>[2x]MDLTNKNVIFVAALGGIGLDTSRELVKRNLKNFVILDRVENPTALAELKAINPKVNITFHTYDVTVPVAE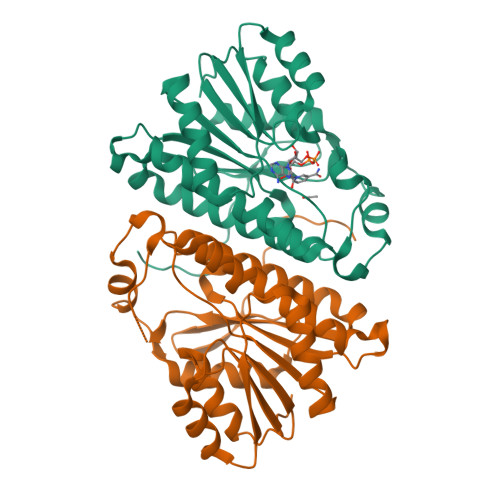SKKLLKKIFDQLKTVDILINGAGILDDHQIERTIAINFTGLVNVTTAILDFWDKRKGGPGGIIANICSVTGFNAIHQVPVYSASKAAVVSFTNSLAKLAPITGVTAYSINPGITRTPLVHTFNSWLDVEPRVAELLLSHPTQTSEQCGQNFVKAIEANKNGAIWKLDLGTLEAIEWTKHWDSHI> AAIGSCSKEYRVLLGQLQKQTDLMQDTSRLLDPYIRIQGLDVPKLREHCRERPGAFPSEETLRGLGRRGFLQTLNATLGCVLHRLADLEQRLPKAQDLERSGLNIEDLEKLQMARPNILGLRNNIYCMAQLLDNSDTAEPTKAGRGASQ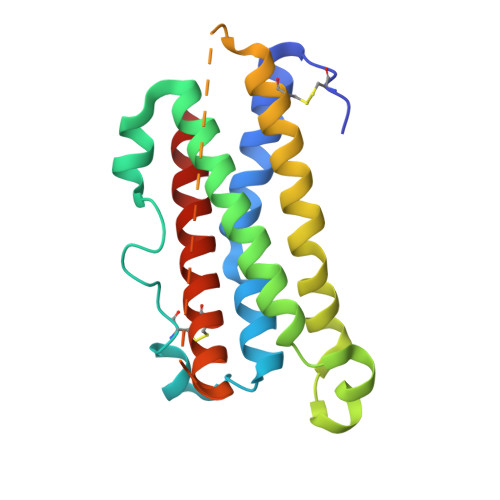PPTPTPASDAFQRKLEGCRFLHGYHRFMHSVGRVFSKW>LVPRGSHMKKLLVANRGEIAVRVFRACNELGLSTVAVYAREDEYSVHRFKADESYLIGQGKKPIDAYLDIDDIIRVALESGADAIHPGYGLLSENLEFATKVRAAGLVFVGPELHHLDIFGDKIKAKAAADEAKVPGIPGTNGAVDIDGALEFAKTYGYPVMIKAALGGGGRGMRVARNDAEMHDGYARAKSEAIGAFGSGEIYVEKYIENPKHIEVQILGDRHGNIIHLHERDCSVQRRNQKVIEIAPAVGLSPDFRNEICEAAVKLCKNVGYVNAGTVEFLVKDDKFYFIEVNPRVQVEHTITELITGVDIVQAQILIAQGKDLHREIGLPAQSEIPLLGSAIQCRITTEDPQNGFLPDTGKIDTYRSPGGFGIRLDVGNAYAGYEVTPYFDSLLVKVCTFANEFSDSVRKMDRVLHEFRIRGVKTNIPFLINVIANENFTSGQATTTFIDNTPSLFNFPRLRDRGTKTLHYLSMITVNGFPGIENTEKRHFEEPRQPLLNLEKKKTAKNILDEQGADAVVDYVKNTKEVLLTDTTLRDAHQSLLATRLRLQDMKGIAQAIDQGLPELFSAEMWGGATFDVAYRFLNESPWYRLRKLRKLMPNTMFQMLFRGSNAVGYQNYPDNVIEEFIRVAAHEGIDVFRIFDSLNWLPQMEKSIQAVRDNGKIAEATICYTGDILDPSRPKYNIQYYKDLAKELEATGAHILAVKDMAGLLKPQAAYRLISELKDTVDLPIHLHTHDTSGNGIITYSAATQAGVDIIDVATASLAGGTSQPSMQSIYYALEHGPRHASINVKNAEQIDHYWEDVRKYYAPFEAGITSPQTEVYMHEMPGGQYTNLKSQAAAVGLGHRFDEIKQMYRKVNMMFGDIIKVTPSSKVVGDMALFMIQNDLTEEDVYARGNELNF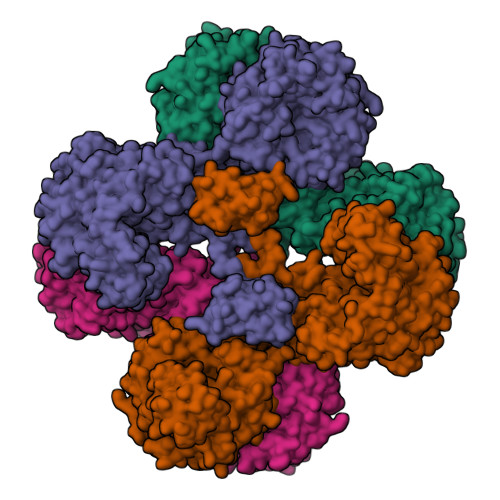PESVVSFFRGDLGQPVGGFPEKLQKIIVKDKAVITDRPGLHAEKVDFETVKADLEQKIGYEPGDHEVISYIMYPQVFLDYQKMQREFGAVTLLDTPTFLHGMRLNEKIEVQIEKGKTLSIRLDEIGEPDLAGNRVLFFNLNGQRREVVINDQSVQAQVVAKRKAETGNPNQIGATMPGSVLEILVKAGDKVQKGQALMVTEAMKMETTIEAPFDGEIVDLHVVKGEAIQTQDLLIEIN[4x]> DPAGLLDLRQGMFAQLVA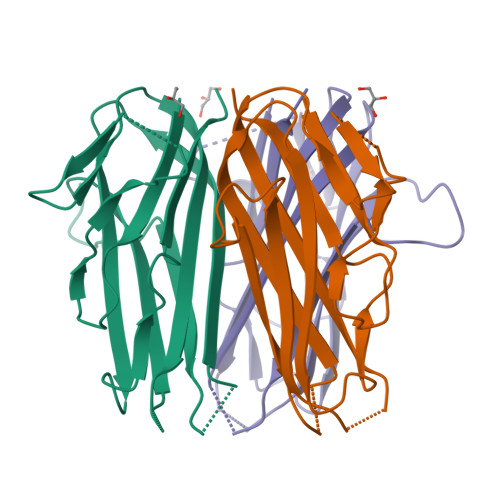QNVLLIDGPLSWYSDPGLAGVSLTGGLSYKEDTKELVVAKAGVYYVFFQLELRRVVAGEGSGSVSLALHLQPLRSAAGAAALALTVDLPPASSEARNSAFGFQGRLLHLSAGQRLGVHLHTEARARHAWQLTQGATVLGLFRVTPEIHHHHHH>GMDYSNELKELFLMNQTYATLFTLTNKIQIEGDKYFGILTSRQYMTILSILHLPEEETTLNNIARKMGTSKQNINRLVANLEKNGYVDVIPSPHDKRAINVKVTDLGKKVMVTCSRTGINFMADVFHEFTKDELETLWSLLK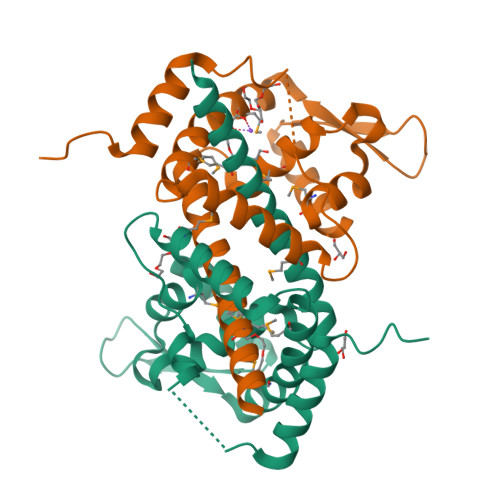KMYRFNGEEQDGFEEDANFMEYEEIDKIKSEALEEFAKRRNRVNKND[2x]> MKVWLVGAYGIVSTTAM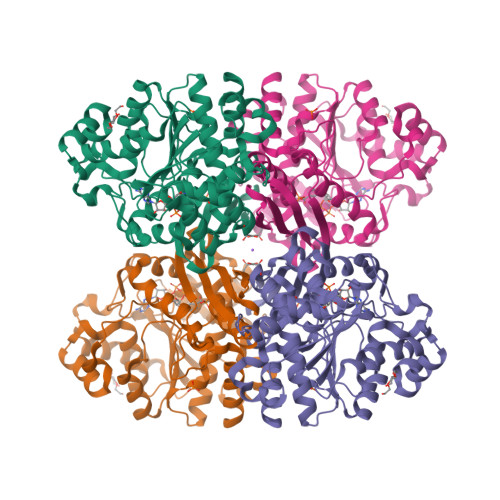VGARAIERGIAPKIGLVSELPHFEGIEKYAPFSFEFGGHEIRLLSNAYEAAKEHWELNRHFDREILEAVKSDLEGIVARKGTALNCGSGIKELGDIKTLEGEGLSLAEMVSRIEEDIKSFADDETVVINVASTEPLPNYSEEYHGSLEGFERMIDEDRKEYASASMLYAYAALKLGLPYANFTPSPGSAIPALKELAEKKGVPHAGNDGKTGETLVKTTLAPMFAYRNMEVVGWMSYNILGDYDGKVLSARDNKESKVLSKDKVLEKMLGYSPYSITEIQYFPSLVDNKTAFDFVHFKGFLGKLMKFYFIWDAIDAIVAAPLILDIARFLLFAKKKGVKGVVKEMAFFFKSPMDTNVINTHEQFVVLKEWYSNLK> CCG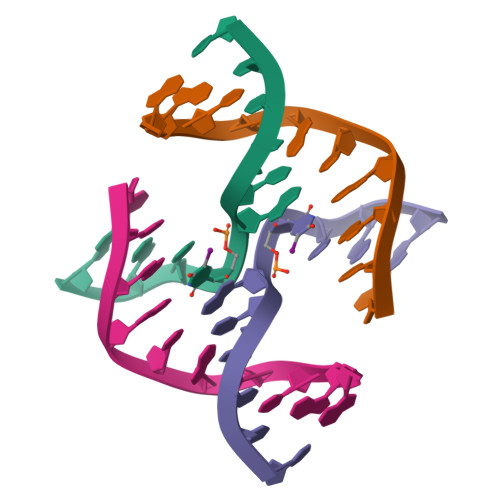GTAUCGG;> CCGATACCGG> DVYQEPTDPKFPQQWYLSGVTQRDLNVKAAWAQGYTGHGIVVSILDDGIEKNHPDLAGNYDPGASFDVNDQDPDPQPRYTQMNDNRHGTRCAGEVAAVANNGVCGVGVAYNARIGGVRMLDGEVTDAVEARSLGLNPNHIHIYSASWGPEDDGKTVDGPARLAEEAFFRGVSQGRGGLGSIFVWASGNGGREHDSCNCDGYT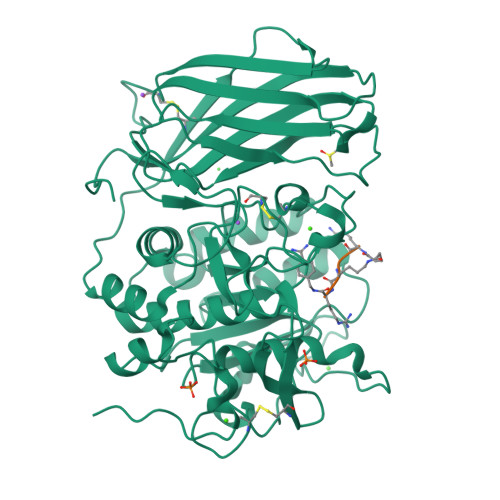NSIYTLSISSATQFGNVPWYSEACSSTLATTYSSGNQNEKQIVTTDLRQKCTESHTGTSASAPLAAGIIALTLEANKNLTWRDMQHLVVQTSKPAHLNANDWATNGVGRKVSHSYGYGLLDAGAMVALAQNWTTVAPQRKCIIDILTEPKDIGKRLEVRKTVTACLGEPNHITRLEHAQARLTLSYNRRGDLAIHLVSPMGTRSTLLAARPHDYSADGFNDWAFMTTHSWDEDPSGEWVLEIENTSEANNYGTLTKFTLVLYGTASGSLVPRGSHHHHHH;> RRKRX2-chloranyl-4-[2-[[(6-chloranyl-1~{H}-indol-2-yl)carbonyl-methyl-amino]methyl]-5-fluoranyl-phenyl]benzoic acid | C24 H17 Cl2 F N2 O3 | 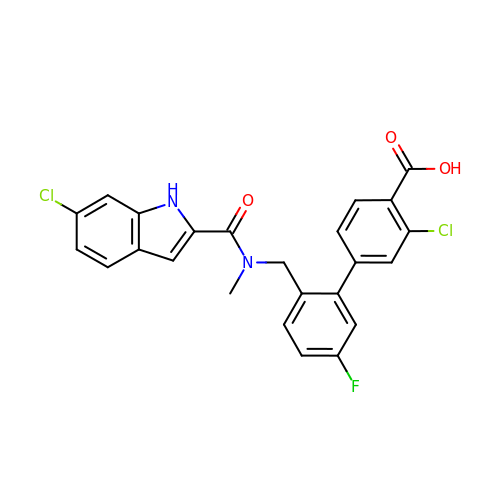QAUQVYLGWNNTGX-UHFFFAOYSA-N> HPETLVKVKDAEDQLGARVGYIELDLNSGKILESFRPEERFPMMGTFKVLLCGAVLSRVDAGQEQLGRRIHYSQNDLVEYSPVTEKHLTDGMTVRELCSAAIT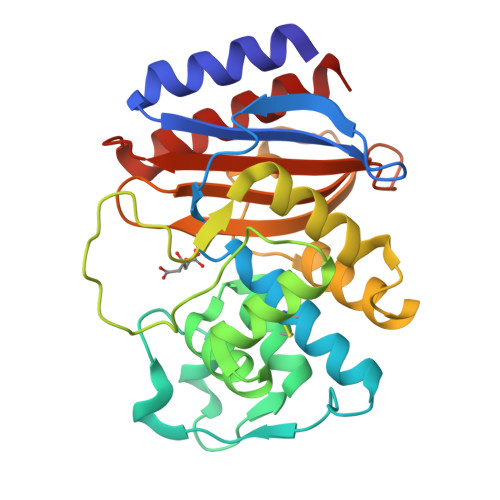MSDNTAANLLLTTIGGPKELTAFLHNMGDHVTRLDRYYGELNEAIPNDERDTTMPAAMATTLRKLLTGELLTLASRQQLIDWMEADKVAGPLLRSALPAGWFIADKSGAGERGSRGIIAALGPDGKPSRIVVIYTTGSQATMDERNRQIAEIGASLIKHW> GSHMAGTMKFKKPPINNPSDDATIKLAEAAVSVSDSMLEMAKVEKVITPPSKDNTLTIPNAYNLQARASVDWSGPIEELTARIAKAAHFRFRVLGKSPSVPVLISISTK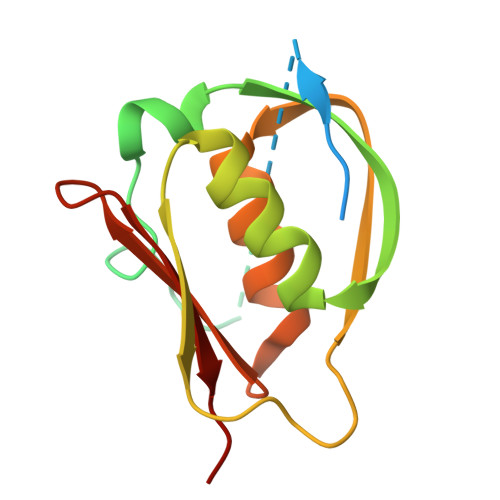DESLAEILRDIDYQAGKKASIHVYPNSQVVELRYAKIYS Here, intermediate forms of the 400 kDa giant Hb from the tubeworm Oligobrachia mashikoi are reported. To overcome the above problems without any artificial modifications to the protein or prosthetic groups, intermediate crystals of the giant Hb were prepared from fully oxygenated crystals by a soaking method. The oxygen saturation of each subunit was determined by occupancy refinement of the bound oxygen based on ambient temperature factors. The structures revealed that local ternary-structural changes are induced at an early stage of oxygen dissociation, and subsequent global ternary-structural changes and large quaternary-structural rearrangement might arise when about half of the oxygen molecules have dissociated from all of the subunits.

Finally, we obtained four crystals with 69%, 58%, 21% and 13% oxygen saturation, designated Crystals 1, 2, 3 and 4, respectively. Crystals 1 and 2 were prepared by the pre-soaking procedure, whereas Crystals 3 and 4 were prepared by the pre-processing procedure. The structures of Crystals 1, 2, 3 and 4 of OliHb were determined at 2.4, 2.7, 2.2 and 2.1 Å resolution, respectively. The average occupancies determined by the B-factor analysis (68%, 51%, 19% and 7.5%) turned out to be slightly lower than the oxygen saturation determined by microspectroscopic analysis for all four crystals. Besides the structural transitions around the heme pockets, the largest ternary-structural changes between the oxy and deoxy form in each subunit are observed in the AB loop region. In Crystal 1, the conformation of the AB loop of the A2 subunit matches that of the deoxy form, whereas the AB loops of the remaining three subunits shows the conformation of the oxy form [Fig. 3(c)]. In Crystals 2, 3 and 4 all of the AB loops show the deoxy conformation. These facts strongly suggest that the AB loop of the A2 subunit is most flexible and most readily transits from the oxy to the deoxy form in the early stages of oxygen dissociation. The side chains of these arginine residues are oriented towards the solvent region in Crystal 1, whereas in Crystals 2, 3 and 4 their orientations are shifted towards the space between His F8 and the heme. The bulky guanidino group would affect the coordination geometry between the heme iron and the proximal His F8, and may reduce the oxygen-binding affinity of the heme.

> VCNRLEQILVKTQWAQSYGEAENRAAFSRDLFSELFNIQGSSRALFSGVGVDDMNSAAFTAHCLRVTGALNRLISQLDQQATINADLAHLAGQHASRNLDASNFAAMGQAVMSVVPTHLDCFNQHAWGECYERIASGISG;> DCTSLNRLLVKRQWAEAYGEGTNRELLGNRIWEDLFANMPDARGLFSRVNGNDIDSSEFQAHSLRVLGGLDMCVASLDDVPVLNALLARLNSQHDSRGIPAAGYPAFVASAISAVRATVGARSFDNDAWNSCMNQIVSGISG;> SSCCSSEDRANVMHNWDAAWSAAYSDRRVALAQAVFASLFSRDAAAQGLFSGVSADNPDSADFRAHCVRVVNGLDVAINMLNDPAVLNEQLAHLSAQHQARAGVAAAHFDVMAEAFAEVMPQVSSCFSSDSWNRCFARIANGISAGL;> ECCSRGDAEVVISEWDQVFNAAMAGSSESAIGVAIFDVFFTSSGVSPSMFPGGGDSSSAEFLAQVSRVISGADIAINSLTNRATCDSLLSHLNAQHKAISGVTGAAVTHLSEAISSVVAQVLPSAHIDAWGYCMAYIAAGIGAGL4-tert-butyl-N-[2-methyl-3-(4-methyl-6-{[4-(morpholin-4-ylcarbonyl)phenyl]amino}-5-oxo-4,5-dihydropyrazin-2-yl)phenyl]benzamide 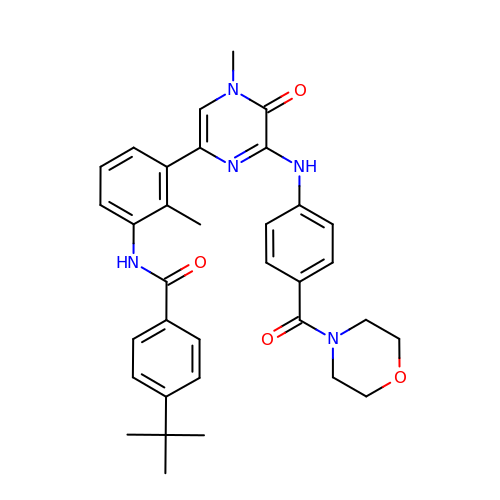| C34 H37 N5 O4 | JIFCFQDXHMUPGP-UHFFFAOYSA-N>IQTTAPPVKESSFVEKMKKTGRNIIVFYGSQTGTAEEFANRLSKDAHRYGMRGMSADPEEYDLADLSSLPEIDKSLVVFCMATYGEGDPTDNAQDFYDWLQETDVDLTGVKFAVFGLGNKTYEHFNAMGKYVDQRLEQLGAQRIFELGLGDDDGNLEEDFITWREQFWPAVCEFFGVEATGEESSIRQYELVVHEDMDVAKVYTGEMGRLKSYENQKPPFDAKNPFLAAVTANRKLNQGTERHLMHLELDISDSKIRYESGDHVAVYPANDSALVNQIGEILGADLDVIMSLNNLDEESNKKHPFPCPTTYRTALTYYLDITNPPRTNVLYELAQYASEPSEQEHLHKMASSSGEGKELYLSWVVEARRHILAILQDYPSLRPPIDHLCELLPRLQARYYSIASSSKVHPNSVHICAVAVEYEAKSGRVNKGVATSWLRAKEPAGENGGRALVPMFVRKSQFRLPFKSTTPVIMVGPGTGIAPFMGFIQERAWLREQGKEVGETLLYYGCRRSDEDYLYREELARFHKDGALTQLNVAFSREQAHKVYVQ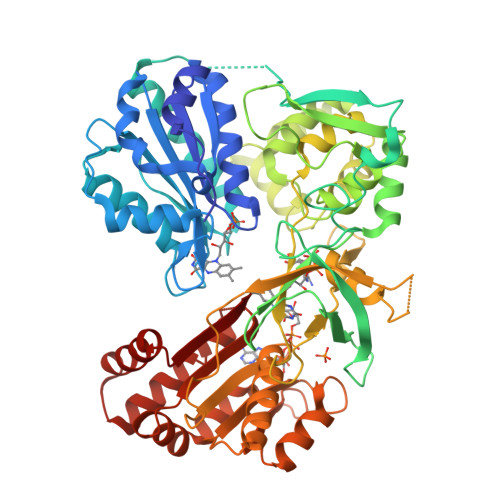HLLKRDREHLWKLIHEGGAHIYVCGAARNMAKDVQNTFYDIVAEFGPMEHTQAVDYVKKLMTKGRYSLDVWS[2x]2-[(2-NAPHTHYLSULFONYL)AMINO]ETHYL DIHYDROGEN PHOSPHATE | C12 H14 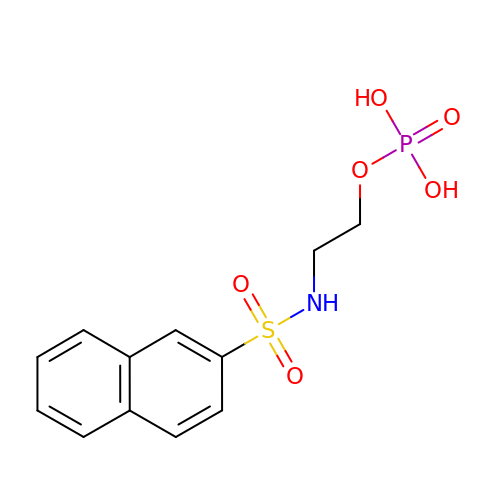N O6 P S | FCROUVVWZFPGFM-UHFFFAOYSA-N>KIPKDTLIIAVENEIARINPAYSEDHDAVINLVFSGLTRFDENMSLKPDLAKSWDISKDGLVYDIFLRDDVLWHDGVKFSADDVKFSIEAFKNPKNNSSIYVNFEDIKSVEILNPSHVKITLFKPYPAFLDALSIGMLPKHLLENENLNTSSFNQNPIGTGPYKFVKWKKGEYVEFKANEHFYLDKVKTPRLIIKHIFDPSIASAELKNGKIDAALIDVSLLNIFKNDENFGILREKSADYRALMFNLDNEFLKDLKVRQALNYAVDKESIVKNLLHDYAFVANHPLERSWANSKNFKIYKYDPKKAEDLLVSAGFKKNKDGNFEKDGKILEFEIWAMSNDPLRVSLAGILQSEFRKIGVVSKVVAKPAGSFDYSKVDSFLIGWGSPLDPDFHTFRV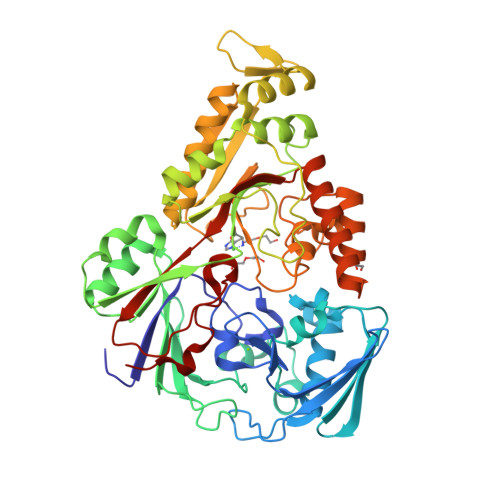FESSQDSALNDEGWNFGHYHDKKVDIALQKARNTSNLEERKKYYKDFIDALYENPPFIFLAYLDFALVYNKDLKGIKTRTLGHHGVGFTWNVYEWSK[2x]> MTDIQLNGKSTLDTPSATMSAKEKEAKLKSADENNKPPNYKRISDSQLYRHSSQYRMWSYTKD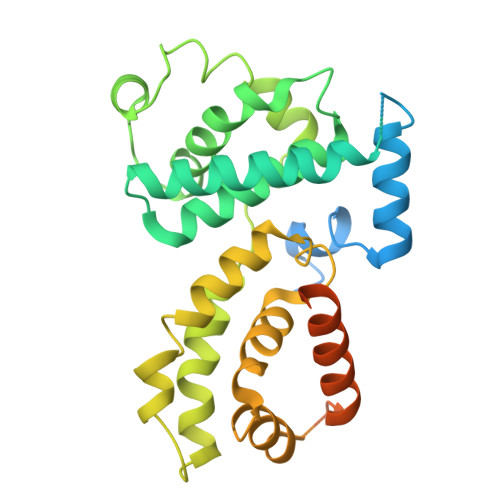QLQEKRVDTNARAIAYIEENLLKFREAHNLTEEEIKVLEAKAIPLTMEEELDLVNFYAKKVQVIAQHLNLPTEVVATAISFFRRFFLENSVMQIDPKSIVHTTIFLACKSENYFISVDSFAQKAKSTRDSVLKFEFKLLESLKFSLLNHHPYKPLHGFFLDIQNVLYGKVDLNYMGQIYDRCKKRITAALLTDVVYFYTPPQITLATLLIEDEALVTRYLETKFPSREGSQESVPGNEKEEPQNDASTTEKNKEKSTESEEYSIDSAKLLTIIRECKSIIEDCKPPSTEEAKKIAAKNYYCQNPSTLIQKLKRKLNGEDTSSTVEKKQKT> GSRATVFKLGLFKSLFLCSFHDITRLFKNDKTTNQQWVLAVFGLAEVFFEASFELLKKQCSFLQMQKRSHEGGTCAVYLICFNTAKSRETVRNLMANMLNVREECLML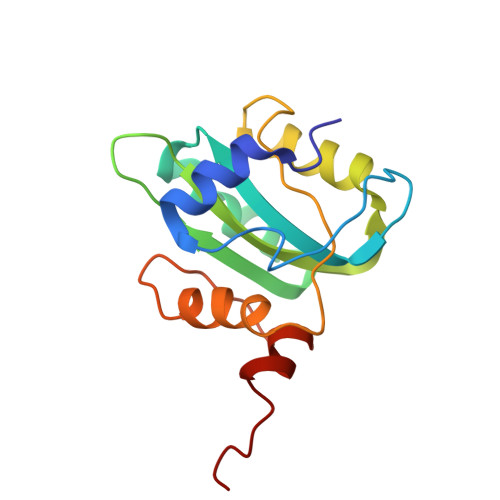QPPKIRGLSAALFWFKSSLSPATLKHGALPEWIRAQTTLNAAAA RNH is a nonspecific endonuclease that degrades RNA within RNA:DNA hybrids. In this study, we traced the evolutionary and mechanistic origins of the thermodynamic differences between mesophilic and thermophilic ribonuclease H1 (RNH) proteins. We then reconstructed ancestral proteins along the evolutionary lineages that connect ecRNH and ttRNH. We observed that, while Tm changed smoothly over both lineages, the mechanism of stabilization followed a more tortuous path.

The other resurrected sequences are evolutionary intermediates at successive phylogenetic nodes along the lineage from Anc1 to ecRNH (AncA through AncD) and from Anc1 to ttRNH (Anc2 and Anc3). Our first goal was to verify that the reconstructed ancestral proteins behaved like members of the RNH family by characterizing their structural and functional properties. Using far-UV CD, we found that all ancestors are folded at 25°C and exhibit secondary structure consistent with extant RNHs. We determined the crystal structure of one representative ancestor, AncC, at 1.3 Å resolution and found that it adopts the canonical RNH fold, superimposing with the ecRNH structure with average Cα RMSD of 0.8 Å and with the ttRNH structure with an average Cα RMSD of 1.3 Å. Finally, we assayed the reconstructed ancestral proteins for their ability to degrade RNA:DNA hybrids using a simple hyperchromic assay to follow RNA cleavage and nucleotide release: all ancestors were active at 25°C, demonstrating that they are all functional ribonucleases H. The temperature-induced unfolding of ancestors along the mesophilic lineage becomes irreversible starting with AncB and continuing through AncC, AncD, and ecRNH. For these proteins, the unfolding curve does not reflect a strictly equilibrium process, so the midpoint of the unfolding curve is therefore only an apparent Tm. AncC and AncD have nearly identical thermostabilities, with Tms ∼7°C lower than Anc1 because of unfavorable changes in ΔHs (−4.4°C) and Ts (−4.3°C) and a favorable change in ΔCp (+1.2°C).

> MLKQVEIFTDGSCLGNPGPGGYGAILRYKQHEKTFSAGFHLTTNNRMELMAAIVALESLKQPCEVILSTDSQYVRQGITQWIHNWKKRGWKTADKKPVKNVDLWQRLDAAIQRHTINWKWVKGHAGHPENERCDELARTAAESPTLEDVGYQPNA1-[4,5-bis(chloranyl)-2,3-dihydroindol-1-yl]ethanone | C10 H9 Cl2 N O | 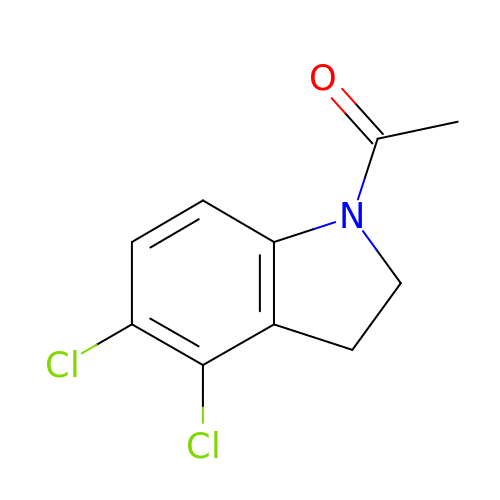FSLARAPYXMNEFP-UHFFFAOYSA-N> MAKKTSSKGKLPPVYPVTVPFLGHIVQFGKNPLEFMQRCKRDLKSGVFTISIGGQRVTIVGDPHEHSRFFSPRNEILSPREVYTIMTPVFGEGVAYAAPYPRMREQLNFLAEELTIAKFQNFVPAIQHEVRKFMAENWKEDEGVINLLEDCGAMIINTACQCLFGEDLRKRLNARHFAQLLSKMESSLIPAAVFMPWLLRLPLPQSARCREARAELQKILGEIIVAREKEEASKDNNTSDLLGGLLKAVYRDGTRMSLHEVCGMIVAAMFAGQHTSTITTSWSMLHLMHPKNKKWLDKLHKEIDEFPAQLNYDNVMDEMPFAERCVRESIRRDPPLLMVMRMVKAEVKVGSYVVPKGDIIA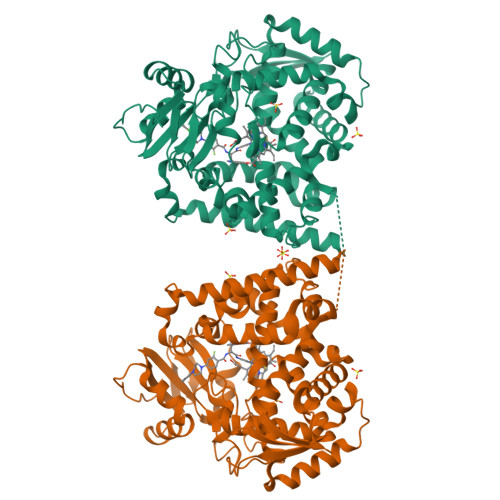CSPLLSHHDEEAFPNPRLWDPERDEKVDGAFIGFGAGVHKCIGQKFALLQVKTILATAFREYDFQLLRDEVPDPDYHTMVVGPTLNQCLVKYTRKKKLPSHHHHHH>MDFSRNLYDIGEQLDSEDLASLKFLSLDYIPQRKQEPIKDALMLFQRLQEKRMLEESNLSFLKELLFRINRLDLLITYLNTRKEEMERELQTPGRAQISAYRVMLYQISEEVSRSELRSFKALLQEEISKCKLDDDMNLLDIFIEMEKRVILGEGKLDI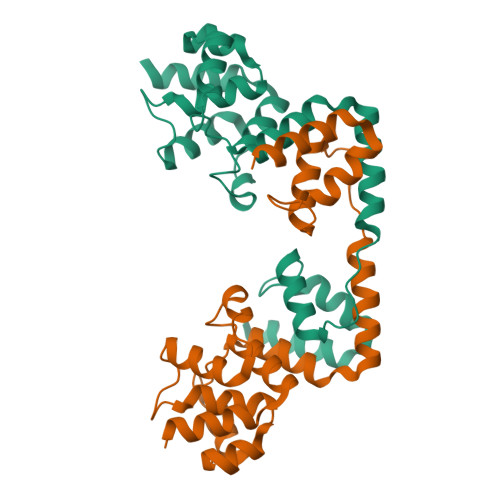LKRVCAQINKSLLKIINDYEEFSKERSSS[2x]Copper-containing nitrite reductases (CuNIRs) catalyze transformation of nitrite to nitric oxide, which has impacts on geochemical, agricultural, and medical health fields. CuNIRs typically have an ∼110 kDa homotrimeric structure, like a Reuleaux triangle. Each protomer contains one type 1 copper (T1Cu) and one type 2 copper (T2Cu) site. The Cys residue forms a peptide-bond bridge (Cys-His bridge) together with one of the His ligands at the T2Cu site to transfer the electron to the catalytic T2Cu site, which is coordinated by three His residues and an axial water molecule.

To further obtain insights into the catalytic intermediates of CuNIR, we performed atomic resolution X-ray crystallography with D98N mutant series of GtNIR in which the Asn residue imitates the protonated state of AspCAT. The structures of D98N without NO2- and C135A/D98N with NO2- were determined at 1.05 and 1.12 Å resolution, respectively. The NO2- complex structure shows multiple conformations of NO2-, indicating that AspCAT is necessary to keep the substrate at the proper position with the configuration suitable for NO2- reduction. In contrast, our atomic resolution data unambiguously revealed three binding modes of NO2-. One is a κ1-O complex that is present only when Asn98 assumes a conformation similar to the gatekeeper (GK) mode. In the GK-like conformation, the side chain of Asn98 is flipped away from the catalytic site and cannot form a hydrogen bond with the substrate. A GK-like conformation of D98N is not observed in the D98N structure without NO2-, which indicates that repulsion between NO2- and Asn98 results in the GK-like conformation. The third binding mode is the κ1-N mode that is also observed in the C135A/D98N structure.

> MESKNKTAATQQSEPNVIAAHKGVNQAPVPLKMERVGPHDVHIEMTAQITDIEIDKGKIYKAWTFNGQAPGPLVVVNEGDTIHFTLKNMDPVVPHSMNFHAVHASPSKDFIDVMPNKSGTFTYPANKPGVFMYHAGTKPVLQHIANGMHGVIIVKPKNGYPTDKEVDREYVLIQNEWYKYNDMNDFQNGVPSYVVFSSKALKPGDPNTNGDTFTLKEKPLLAKVGEKIRLYINNVGPNEVSSFHVVGTVFDDVYLDGNPNNHLQGMQTVMLPASGGAVVEFTVTRPGTYPIVTHQFNHAQKGAVAMLKVTETGEDDGTETSGH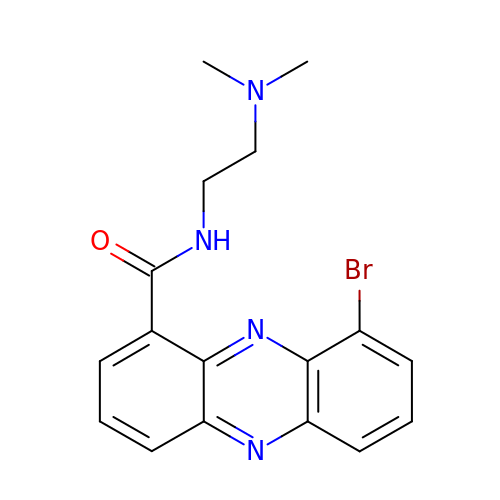9-BROMO-PHENAZINE-1-CARBOXYLIC ACID (2-DIMETHYLAMINO-ETHYL)-AMIDE | C17 H17 Br N4 O | QCANCQNKYBFYAC-UHFFFAOYSA-N>[2x]SNAMRRNEDSWLIDGATPLEDVMRALNIH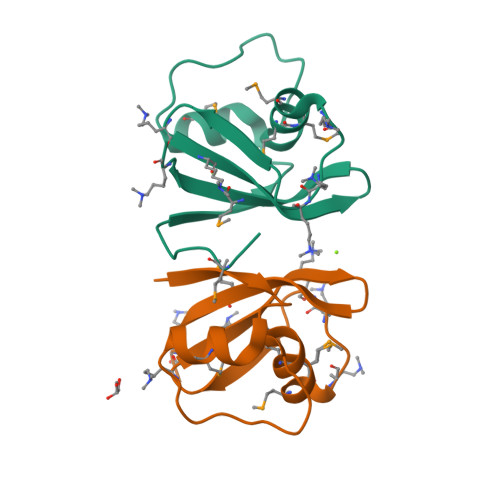TFPRDENYETIGGFMMYMLRKIPKKTDFVLYDKYKFEIIDTENFRIDQLMVSFRKDV N'-[(1S,2R)-2-[(2R,4R)-4-(BENZYLOXY)PYRROLIDIN-2-YL]-1-(3,5-DIFLUOROBENZYL)-2-HYDROXYETHYL]-5-METHYL-N,N-DIPROPYLISOPHTHALAMIDE 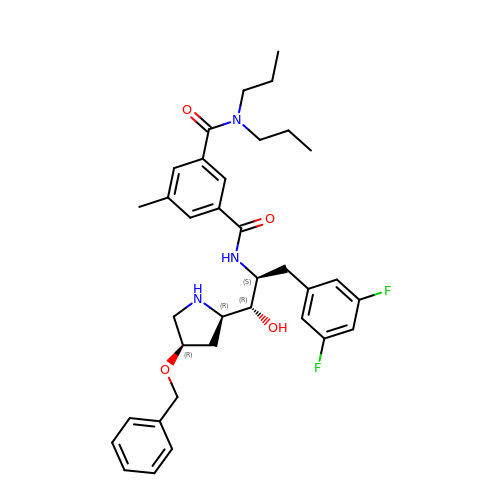| C35 H43 F2 N3 O4 | GZHSLBYVXGDJDF-NXVJRICRSA-N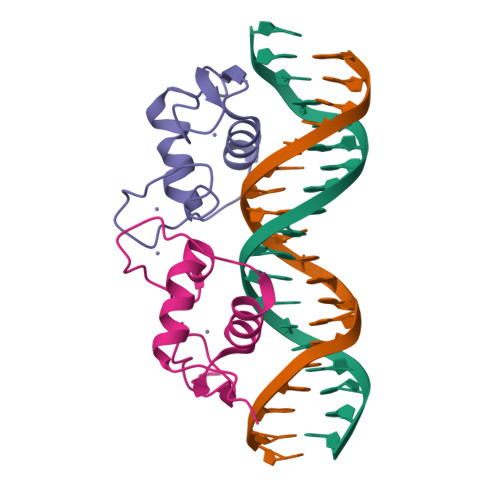>[2x]MKPARPCLVCSDEASGCHYGVLTCGSCKVFFKRAVEGQHNYLCAGRNDCIIDKIRRKNCPACRYRKCLQAGMNLEARKTKKKIKGIQQATAG>GMTTPRRALIVIDVQNEYVTGDLPIEYPDVQSSLANIARAMDAARAAGVPVVIVQNFAPAGSPLFARGSNGAELHPVVSERARDHYVEKSLPSAFTGTDLAGWLAARQIDTLTVTGYMTHNCDASTINHAVHSGLAVEFLHDATGSVPYENSAGFASAEEIHRVFSVVLQSRFAAVA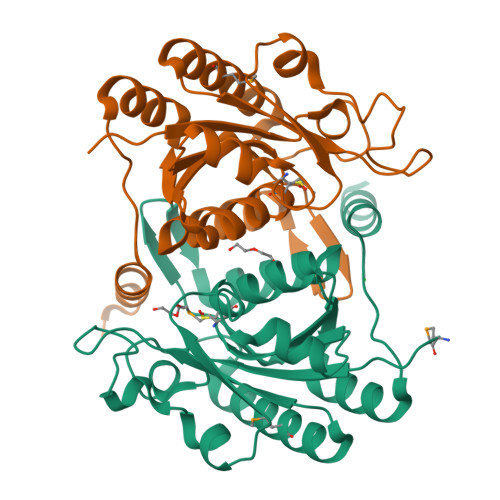STDEWIAAVQGGTPLARGNIYASNQKARARRATA[2x]> MAHHHHHHVDDDDKMLEVLFQGPEAPVLMMATTTSTDNTGLLDDLAPQFTKDTGIELRWTAVGTGKALKMGENCDVDILLVHAPAAEKAFVDAGFGTARTQLMYNDFVIIGPAADPAGVKGMTVAAALGKIAADNAVFVSRGDNSGTHKMEKSLWKQIEGPSP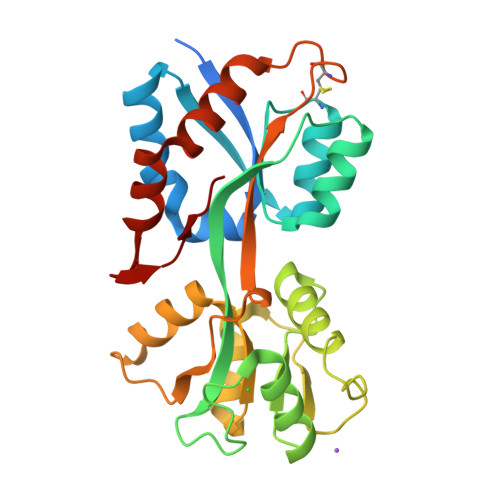EKEAWYVQTGQGMLRTINVAAEKGGYTMTDRGTYIKYEASMDGNPPLKILVEGDKILFNQYSAIPVNPAHCPKVKKDLADKFVNWMASPATQKTIGDFKLMGKALFTPNAE>[4x]MEYRYDDNATNVKAMKYLIEHYFDNFKVDSIEIIGSGYDSVAYLVNNEYIFKTKFSTNKKKGYAKEKAIYNFLNTNLETNVKIPNIEYSYISDELSILGYKEIKGTFLTPEIYSTMSEEEQ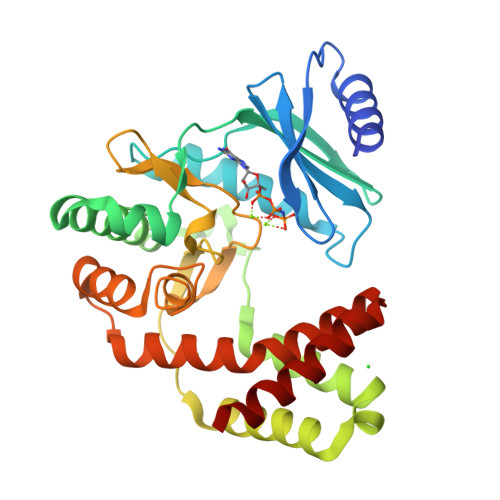NLLKRDIASFLRQMHGLDYTDISECTIDNKQNVLEEYILLRETIYNDLTDIEKDYIESFMERLNATTVFEGKKCLCHNDFNCNHLLLDGNNRLTGIIDFGDSGIIDEYCDFIYLLEDSEEEIGTNFGEDILRMYGNIDIEKAKEYQDIVEEYYPIETIVYGIKNIKQEFIENGRKEIYKRTYKD> MEGMRRPTPTVYVGRVPIGGAHPIAVQSMTNTPTRDVEATTAQVLELHRAGSEIVRLTVNDEEAAKAVPEI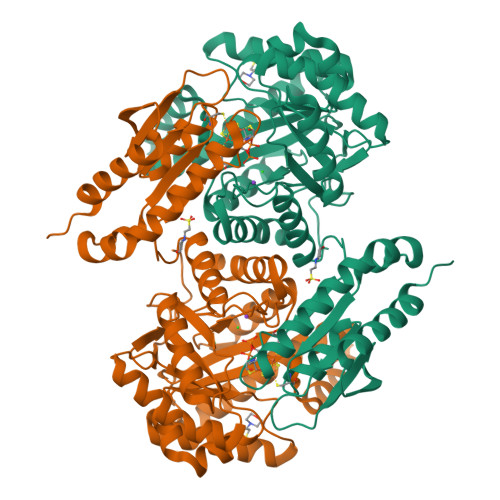KRRLLAEGVEVPLVGDFHFNGHLLLRKYPKMAEALDKFRINPGTLGRGRHKDEHFAEMIRIAMDLGKPVRIGANWGSLDPALLTELMDRNASRPEPKSAHEVVLEALVESAVRAYEAALEMGLGEDKLVLSAKVSKARDLVWVYRELARRTQAPLHLGLTEAGMGVKGIVASAAALAPLLLEGIGDTIRVSLTPSPKEPRTKEVEVAQEILQALGLRAFAPEVTSCPGCGRTTSTFFQELAEEVSRRLKERLPEWRARYPGVEELKVAVMGCVVNGPGESKHAHIGISLPGAGEEPKAPVYADGKLLTILKGEGIAEEFLRLVEDYVKTRFAPKA>[2x]MEQEKVQELVSQMTLDEKIAQCLQLSPFLFKGTNKNAELTGPLLQEMKLTDAHTENAGSVLGSSSALDMIGIQEAYLKTNRLGIPLVFMADVIHGYKTVFPIPLALGCSFDRETVRVMAEVSALEATADGHHVTFSPMLDLVRDPRWGRVMESTGEDPFLNSELGKAMVDGYQGDASKLNENLEQMAACVKHFAAYGAAEAGLEYNTVNMSTRELYQNYLPAYNAAIQAGAKLVMTAFNVVDGIPATMNKWLNRDVLRGEMEFDGVLISAWGA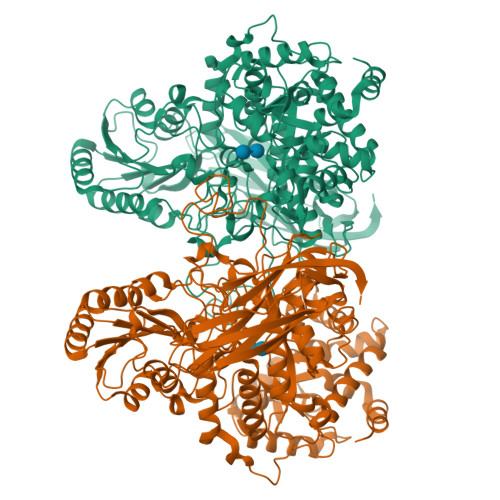VAEVINHGTARNPKEAAQFSMEAGVDLEMMTTCYIHELKGLIEEGKLSENLLDEAVLRMLNLKNDLGLFEDPYRGLKNNDRTKDILTDESRGKARAAGVESAVLLENKSRLLPLAKEAKIALVGPLATSPDILGGWNVYGEEKDGINVETGLREVFETVEVVSTEYTELSEEDKVAVKAAVQNMDVVVLALGEKNEWGGEAGSLATIRLPEAQYQLAKFVQTLGKPVVITLFNGRPLEVKELAESSDALLELWFPGTEAGRVTADLLSGASNPSGKLSMSFPQTTGQIPVYYNHLRTGRPQTPENKGERYVSHYLDIPNEPFYPFGYGKSYSEFELKTSSLPKELNLGESLHVEVTIKNISDIAGKEVIQVYLQDVTASISRPVKELKAFEKVALQAGEEKTVTFELTSEAFSFYNHQLEKVQEPGLHRVFVGTSSEDVDVFEVEVGGYVLEHHHHHH>HHHHHHMATFTTEQAGYQMQAILQVIGYDLLIVVTGGTNPHIGDVTTLTASTVPETVKFPSHDGRFHKDNFISERMAKRIQRYLAGSCTITAGIHVNQITKAQIAAAAPMTDDLSRQIISWLQAHPVQAEKPEYYGQDEQPR[2x]

Previous studies indicated that the small protein LpdD (lp_0272) is associated with the UbiD-type gallate decarboxylase LpdC (lp_2945) in Lactobacillus plantarum. The crystal structure of the purified LpdD reveals a dimeric protein with structural similarity to the eukaryotic heterodimeric proteasome assembly chaperone Pba3/4. Solution studies demonstrate that LpdD protein specifically binds to reduced prFMN species only. The addition of the LpdD–prFMNH2 complex supports reconstitution and activation of the purified E. coli apo-UbiD in vitro, leading to modest 3,4-dihydroxybenzoic acid decarboxylation. These observations suggest that LpdD acts as a prFMNH2-binding chaperone, enabling apo-UbiD activation through enhanced prFMNH2 incorporation and subsequent oxidative maturation.

Despite multiple attempts, the crystal structure of LpdD in complex with prFMNH2 could not be determined, because of the difficulties associated with maintaining the strict anaerobic conditions required. However, LpdD crystals soaked with MnCl2 and prFMNH2 did reveal the presence of a metal ion in the electron density, coordinated by His35, His61, and Asp63 residues. Major conformational changes were observed when compared with the non–metal-bound apo-LpdD in the F53–I66 loop region, containing two of the three ligating residues. This region is highly conserved despite having no obvious structural role in the apo-LpdD, which may indicate Mn2+ binding could be relevant for activity, as is observed for UbiD enzymes. Structure elucidation reveals LpdD is similar in structure to a eukaryotic chaperone involved in 20S proteosome assembly, with a highly conserved region exposed at the protein surface. The latter includes a metal-binding site with possible relevance to function, with the conserved H35–H61–D63 providing a Mn2+-binding site. The coordination pattern allows a fourth nonprotein ligand to bind, possibly the prFMN phosphate when in complex with the cofactor, thus resembling the UbiD Mn2+-assisted prFMN binding. The presence of MnCl2 (Mn2+ is required for prFMN binding in UbiD but not UbiX) in the reconstitution buffer appears to have no noticeable effect on LpdD–prFMNH2 binding. Furthermore, WT LpdD prFMNH2 binding occurs in the absence of Mn2+, which suggests metal binding is not essential for activity. Given the LpdD conserved surface–exposed region largely consists of loop regions that are shown to alter conformation in response to either metal binding or single-site mutations, we suggest that the LpdD–prFMNH2 complex likely has a distinct conformation through induced fit binding, hindering accurate modeling of the complex on the basis of the non–cofactor-bound structures.> G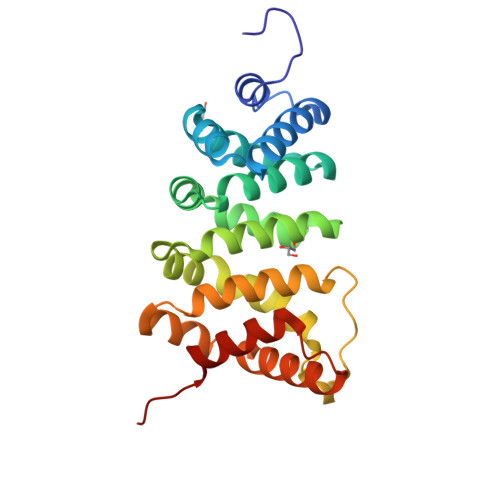SNADMEMTLERAVSMLEADHMLPSRISAAATFIQHECFQKSEARKRVNQLRGILKLLQLLKVQNEDVQRAVCGALRNLVFEDNDNKLEVAELNGVPRLLQVLKQTRDLETKKQITGLLWNLSSNDKLKNLMITEALLTLTENIIIPFSGWPEGDYPKANGLLDFDIFYNVTGCLRNMSSAGADGRKAMRRCDGLIDSLVHYVRGTIADYQPDDKATENCVCILHNLSYQLEA> GSENIYTTLKFESMMQQRVIQIRSIPEEEYHELVSVQFKTDGGKYEKGEKQDLELSEKKTENGKDTESWGWNENQDSDEHDGWDEELDIDVD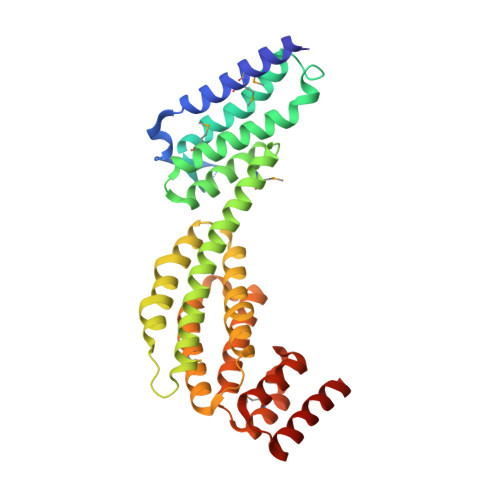NVPIQVSVFVQSAAKVFTEFEQGCDTIGRSKVESIYLYKFNLLQTAFFAMVSEKVNDWTQLYKDVRYLYTENPKLLQLMELNSRRLDLNLNLIKKTIYKLVNDQLQELKDNERTPDWDITISSLLPYLKKTALPTLYKLEDNTILVALIRYIVHDLVIDNILHWRVISEKSSENLSEFIMLLLSGLEIPRLNLIETYRHSREKLGILSKILTAHLKDILEMFYEGEFFLFETDEIVQWIILLFADTPTRRDCIDEIRRVREEATD2-[4-[(2~{R},4~{S})-4-phenylpyrrolidin-2-yl]carbonylpiperazin-1-yl]pyridine-3-carbonitrile | C21 H23 N5 O | 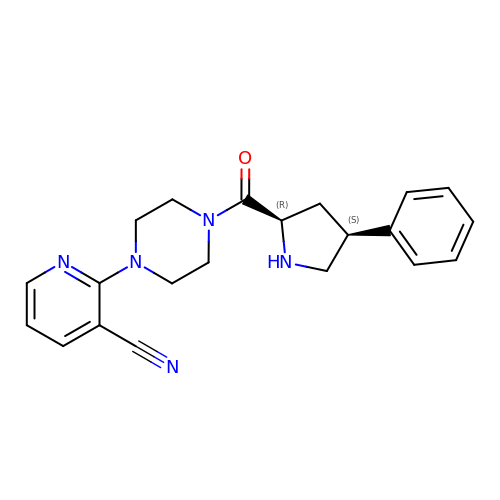ZOCRTPMGIHWFKT-RTBURBONSA-N>[3x]KPATAARATGLADFKPGVQWEICIHHPIKHDSAADLIPTKAKVWDIDMGHAQEFPNMIPMLKSAGKFVICYFNAGALQDWDDDKSKFPKEVIGHSLSYPYDSEEWYLDIRDSRVLELQTARLDIAAKIGCDAVDPDNVDAWQQDDEDPTGFKLKSSDYTNYLKNLAKYAHSIKTKDGQPLLVGQKNAPEIAEDLVSTLDFAVLESCRGNSDPNEESWPFCEDFQTYIDAGKPVLQIEYPPSVEKTGKVSASDNKYYCTAEDEDKGFSKIIKWASAQLDGWGQYCGEEPFRTPAAKY

Endo-galactosaminidases are an underexplored family of enzymes involved in the degradation of galactosaminogalactan (GAG) and other galactosamine-containing cationic exopolysaccharides produced by fungi and bacteria. Whereas the fungal enzyme belongs to family GH114, the two bacterial enzymes do not lie in the current GH families but instead define a new family, GH191. The TIM-barrel core structure with fully conserved active-site residues and a negatively charged substrate crevice is conserved among all the families. The putative active-site residues (Asp156/Glu225 for TmGH191, Asp323/Glu391 for Env-GH191 and Asp157/Glu225 for FsGH114) overlap well with the experimentally verified nucleophile and general acid/base Asp189/Glu247 in Ega3, Asp196/Glu222 in Sph3 and Asp160/Glu223 in PelAH.

The fungal GH114 enzyme from the filamentous fungus F. solani, which shows a sequence identity of 33% to Ega3 from A. fumigatus, could also be produced in soluble form. For FsGH114 no activity was seen using the isolated Pel substrate and further studies are necessary to establish the exact substrate specificity of FsGH114. Similarly, within the GH114 family, F. solani GH114 overlaps with Ega3 (AfGH114) with an r.m.s.d. of 1.49 Å over 218 residues, with a sequence identity of 35%. FsGH114 also lacks the first and sixth α-helices but has a C-terminal extension folding into two strands forming a short antiparallel β-sheet. One of these tyrosines or both could play the same role as the tryptophans in the other three enzymes (Tyr121 is poorly defined in the present structure). The acceptor side of the substrate crevice in FsGH114 is flanked by two elongated loops comprising residues 164–168 between β4 and α4 and C-terminal to β6 residues 231–239. Thus, overall the crevice of FsGH114 is deeper and more pronounced compared with the bacterial GH191 enzymes, but also with Ega3. To gain better insight into the substrate interactions, we docked the substrate into Env-GH191 and FsGH114. In both cases up to seven subsites could be identified. Whereas the Env-GH191 binding crevice seem to better fit the galactosamine oligomer, the FsGH114 crevice can accommodate either an acetylated or a non-acetylated GAG oligomer equally well.N-{[(4-methylphenyl)carbonyl]carbamoyl}-beta-D-glucopyranosylamine 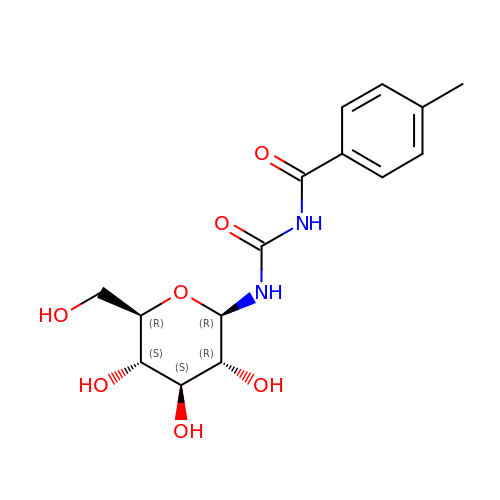| C15 H20 N2 O7 | DUVVGYBLYHSFMV-YGEZULPYSA-N> MASVHGTTYELLRRQGIDTVFGNPGSNELPFLKDFPEDFRYILALQEACVVGIADGYAQASRKPAFINLASAAGTGNAMGALSNAWNSHSPLIVTAGQQTRAMIGVEALLTNVDAANLPRPLVKWSYEPASAAEVPHAMSRAIHMASMAPQGPVYLSVPYDDWDKDADPQSHHLFDRHVSSSVRLNDQDLDILVKALNSASNPAIVLGPDVDAANANADCVMLAERLKAPVWVAPSAPRCPFPTRHPCFRGLMPAGIAAISQLLEGHDVVLVIGAPVFRYHQYDPGQYLKPGTRLISVTCDPLEAARAPMGDAIVADIGAMASALANLVEESSRQLPTAAPEPAKVDQDAGRLHPETVFDTLNDMAPENAIYLNESTSTTAQMWQRLNMRNPGSYYFCAAGGLGFALPAAIGVQLAEPERQVIAVIGDGSANYSISALWTAAQYNIPTIFVIMNNGTYGALRWFAGVLEAENVPGLDVPGIDFRALAKGYGVQALKADN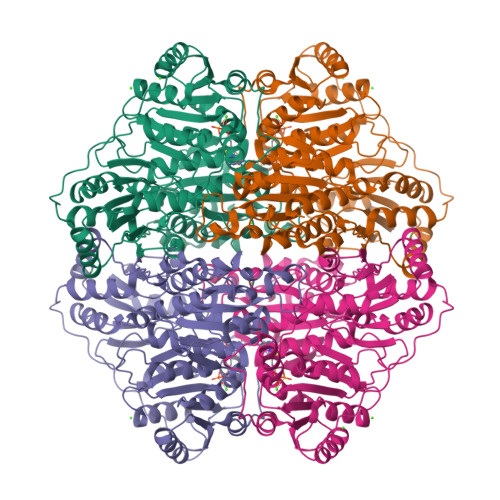LEQLKGSLQEALSAKGPVLIEVSTVSPVKRSHHHHHH> MSDLEQLKQILGNGLTDQTFLLEPRTGKGLL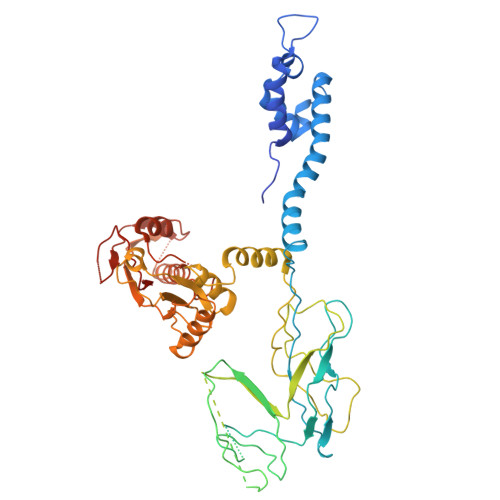NLMAKYTEAVPFAGHTDADWKDFWMAGCTLEALSDIYQYPGLAEKKLPVQQAFLLALLHLLETPRAMLNTVPARHRSLYYRDLLGFAPRAPQPDSVAVSFTLQRNSSPYALPAGSLLDGGQDSAGNSITYQTDDSLLITGQQLEQLCWTAQVGETWKRYTAIDSATGVTLPAEGLRLFTATGQGTDTKEKAPELYLGFSGTSAQDTLSLYWSVRASSALDVTWWYYQGTKWASLDAELQDNTASLSVSNLWRARLPADSQPGSGLPQDDEPLEAGYYWIKGTLKENKEAKDENSPAEAMPQLQAVLANAMTATLNVAQAIDDSHFSQPLPANTINQLVTPVAAISDVRQPLPSVGGQPRETEMAMLQRAAPRIAHRQRAITWNNMRSLLMEHYPEIFDVRFPDVDKLSRLPALEVQSLMVIPDGRYGDNDDALRPALSNGRLSRMAQWLSQYTSLWAAPTLKNPKYIDVTARYRVTFVVGIRPDYGYRQLAAQLQHDYMPWATDRRQAVTPGNQVDYYQLLATLQQSPLVQSVNALVLSHDVIDETGKPTSMETQSTVTARDDEVLILCPEGETHV>AKVFQWFGSNESGAEFGSQNLPGVEGKDYIWPDPNTIDTLISKGMNIFRVPFMMERLVPNSMTGSPDPNYLADLIATVNAITQKGAYAVVDPHNYGRYYNSIISSPSDFQTFWKTVASQFASNPLVIFDTNNQYHDMDQTLVLNLNQAAIDGIRSAGATSQYIFVEGNSWTGAWTWTNVNDNMKSLTDPSDKIIYEMHQFLDSDGSGTSATCVSSTIGQERITSATQWLRANGKKGIIGEFAGGANDV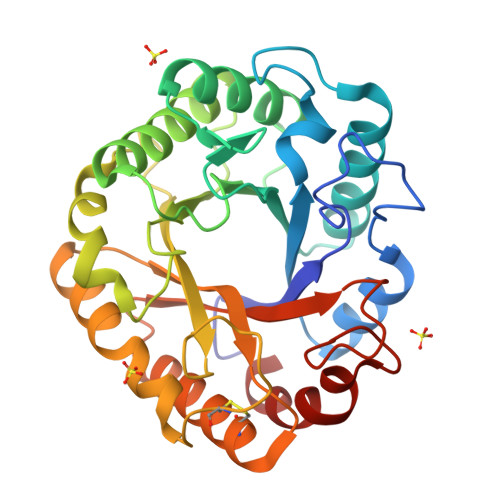CETAITGMLDYMAQNTDVWTGAIWWAAGPWWGDYIFSMEPDNGIAYQQILPILTPYL[2x]> STGSATTTPIDSLDDAYITPVQIGTPAQTLNLDFDTGSSDLWVFSSETTASEVDGQTIYTPSKSTTAKLLSGATWSISYGDGSSSSGDVYTDTVSVGGLTVTGQAVESAKKVSSSFTEDSTIDGLLGLAFSTLNTVSPTQQKTFFDNAKASLDSPVFTADLGYHAPGTYNFGFIDTTAYTGSITYTAVSTKQGFWEWTSTGYAVGSGTFKSTSIDGIADTGTTLLYLPATVVSAYWAQVSGAKSSSSVGGYVFPCSATLPSFTFGVGSARIVIPGDYI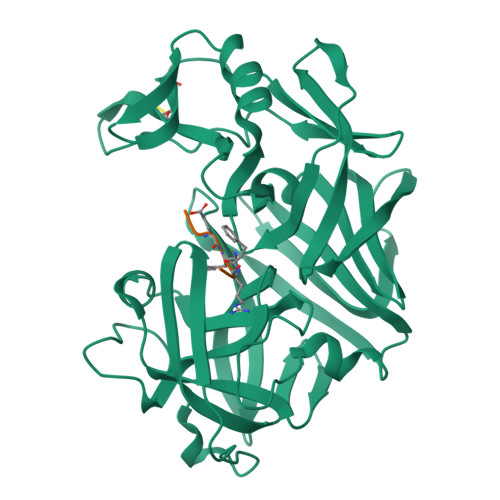DFGPISTGSSSCFGGIQSSAGIGINIFGDVALKAAFVVFNGATTPTLGFASK;> PTEXRE4-acetylpiperazine-1-carboxamide | C7 H13 N3 O2 | 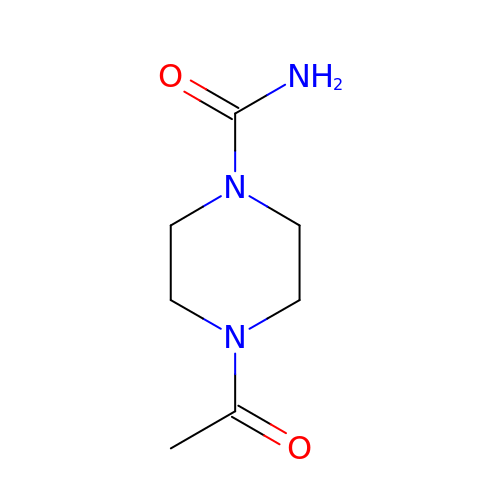DBVCCTKTVHHAAW-UHFFFAOYSA-N>[2x]LGSSNDNIELVDFQNIMFYGDAEVGDNQQPFTFILDTGSANLWVPSVKCTTAGCLTKHLYDSSKSRTYEK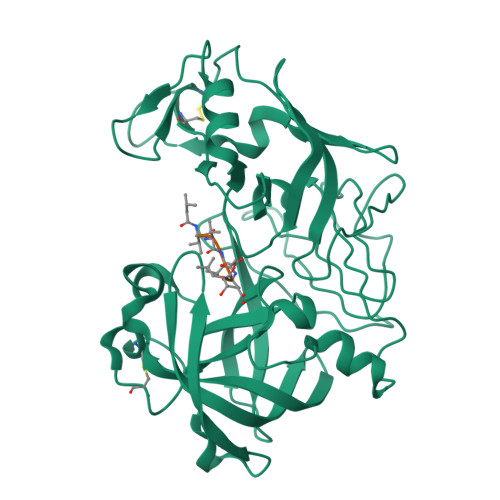DGTKVEMNYVSGTVSGFFSKDLVTVGNLSLPYKFIEVIDTNGFEPTYTASTFDGILGLGWKDLSIGSVDPIVVELKNQNKIENALFTFYLPVHDKHTGFLTIGGIEERFYEGPLTYEKLNHDLYWQITLDAHVGNIMLEKANCIVDSGTSAITVPTDFLNKMLQNLDVIKVPFLPFYVTLCNNSKLPTFEFTSENGKYTLEPEYYLQHIEDVGPGLCMLNIIGLDFPVPTFILGDPFMRKYFTVFDYDNHSVGIALAKKNL propyl (3~{S})-4-[[(6~{R})-6-(aminomethyl)-5,6,7,8-tetrahydroacridin-3-yl]carbonyl]-3-methyl-piperazine-1-carboxylate | C24 H32 N4 O3 | 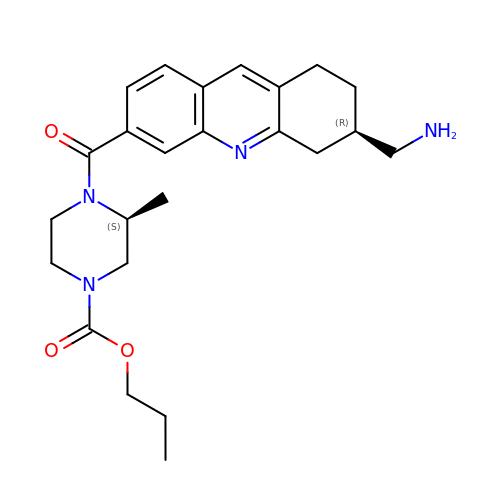SKXOWPNKAZGYJW-DLBZAZTESA-N>[2x]GLYVGGFVDVVSCPKLEQELYLDPDQVTDYLPVTEPLPITIEHLPETEVGWTLGLFQVSHGIFCTGAITSP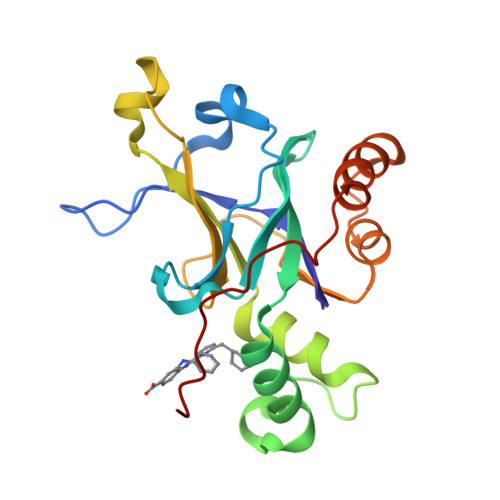AFLELASRLADTSHVARAPVKNLPKEPLLEILHTWLPGLSLSSIHPRELSQTPSGPVFQHVSLCALGRRRGTVAVYGHDAEWVVSRFSSVSKSERAHILQHVSSCRLEDLSTPNFVSPLETL BMP-9 and BMP-10 are TGF-β family signaling ligands naturally secreted into blood. They act on endothelial cells and are required for proper development and maintenance of the vasculature. BMP-9 and −10 are synthesized as pro-proteins and processed by furin to release growth factors comprised of two cystine-knotted protomers that can covalently homo- or hetero-dimerize via a single cysteine in the dimer interface. Unlike other ligands of the TGF-β family, BMP-9 and −10 are secreted as a mixture of disulfide-linked dimers and monomers, in which the interchain cysteine (Cys-392) remains either paired or unpaired.

To further understand how these residues contribute to growth factor dimerization, BMP-9 G389S and BMP-9 G389S, K357R disulfide-linked dimers were crystallized at both neutral and low pH. For BMP-9 dimer mutants at neutral pH, the well solution was 1M NaCl, 22–26% glycerol, 0.1 M HEPEs pH 7.4, and the cryoprotectants ranged across 25–35% glycerol. For the crystals where the datasets were split, the integrated diffraction data was split using rebatch in the CCP4 suite to take either the first or last 32nd (or first 64th for wild type BMP-9) of diffraction images from each crystal’s 360° datasets. Where the serine is present, its sidechain hydroxyl is unstructured at neutral pH. Where the arginine is present, the sidechain guanidino group sits between the serine and predicted backbone oxygen contact at the edge of accepted hydrogen bonding distances. Since wild type BMP-9 is radiation sensitive, the BMP-9 mutants were checked for radiation sensitivity. At neutral pH, the mutants lost density due to radiation damage but remained disulfide bonded. While neither mutant’s disulfide could be unambiguously modeled in a strained conformation, the radiation sensitivity demonstrates that the bonds are not ideal. While the trend is not clear between mutants at neutral pH, the damage is decreased compared to wild-type. Similarly, the double mutants further improve BMP-9 disulfide bond formation but fail to further impair BMP-10 disulfide bond formation.

> SSGAGSHCQKTSLRVNFEDIGWDSWIIAPKEYEAYECRGGCFFPLADDVTPTKHAIVQTLVHLKFPTKVSKACCVPTKLSPISVLYKDDMGVPTLKYHYEGMSVAECGCR> MENTENSVASKSIKNLEPKIIHGSESMASGISLDNSYKMDYPE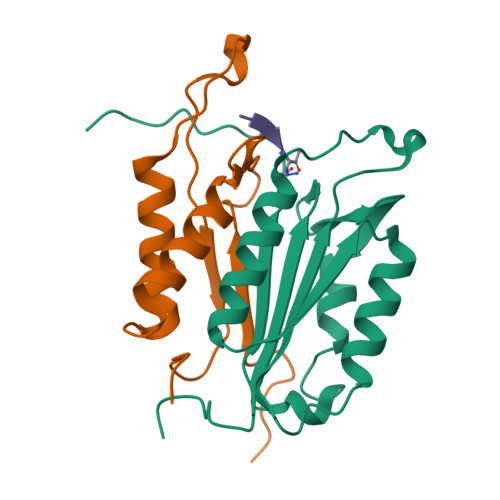MGLCIIINNKNFHKSTGMTSRSGTDVDAANLRETFRNLKYEVRNKNDLTREEIVELMRDVSKEDHSKRSSFVCVLLSHGEEGIIFGTNGPVDLKKITNFFRGDRCRSLTGKPKLFIIQACRGTELDCGIETD;> SGVDDDMACHKIPVEADFLYAYSTAPGYYSWRNSKDGSWFIQSLCAMLKQYADKLEFMHILTRVNRKVADEFESFSFDATFHAKKQIPCIVSMLTKELYFYH>ATDRGSESDKHFRKVSDKEKIDQLQEELLHTQLKYQRILERLEKENKELRKLVLQKDDKGIHHRKLKKSLIDMYSEVLDVLSD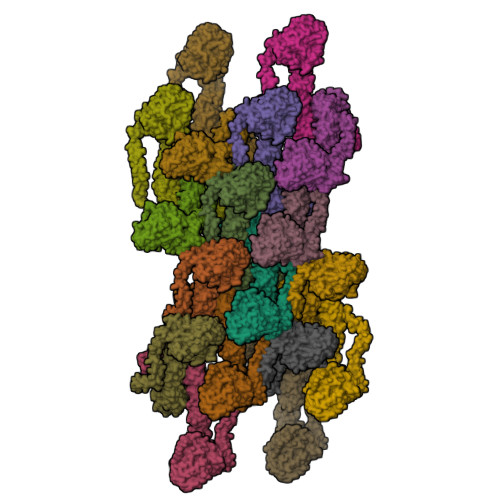YDASYNTQDHLPRVVVVGDQSAGKTSVLEMIAQARIFPRGSGEMMTRSPVKVTLSEGPHHVALFKDSSREFDLTKEEDLAALRHEIELRMRKNVKEGCTVSPETISLNVKGPGLQRMVLVDLPGVINTVTSGMAPDTKETIFSISKAYMQNPNAIILCIQDGSVDAERSIVTDLVSQMDPHGRRTIFVLTKVDLAEKNVASPSRIQQIIEGKLFPMKALGYFAVVTGKGNSSESIEAIREYEEEFFQNSKLLKTSMLKAHQVTTRNLSLAVSDCFWKMVRESVEQQADSFKATRFNLETEWKNNYPRLRELDRNELFEKAKNEILDEVISLSQVTPKHWEEILQQSLWERVSTHVIENIYLPAAQTMNSGTFNTTVDIKLKQWTDKQLPNKAVEVAWETLQEEFSRFMTEPKGKEHDDIFDKLKEAVKEESIKRHKWNDFAEDSLRVIQHNALEDRSISDKQQWDAAIYFMEEALQARLKDTENAIENMVGPDWKKRWLYWKNRTQEQCVHNETKNELEKMLKCNEEHPAYLASDEITTVRKNLESRGVEVDPSLIKDTWHQVYRRHFLKTALNHCNLCRRGFYYYQRHFVDSELECNDVVLFWRIQRMLAITANTLRQQLTNTEVRRLEKNVKEVLEDFAEDGEKKIKLLTGKRVQLAEDLKKVREIQEKLDAFIEALHQEK[18x]3-[4-(benzyloxy)phenyl]propan-1-ol | C16 H18 O2 | 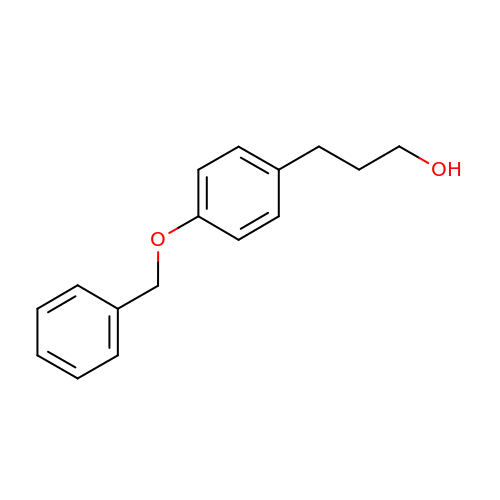FZALPKMIIYFLAP-UHFFFAOYSA-N> MSEQDEVPSEDRRKYEFRKVIEELKDYEGSGTQLVTIYI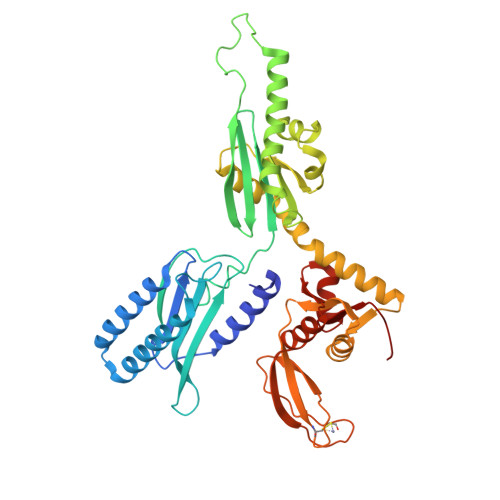PPDKQISDVVAHVTQEHSEASNIKSKQTRTNVQDALTSIKDRLRYYDTFPPDNGMVVFSGAVDSGGGRTDMVTEVLESPPQPIESFRYHCDSAFLTEPLAEMLGDKGLYGLIVLDRRESNVGWLKGKRVQPVKSAESLVPGKQRKGGQSAQRFARLRLEAIDNFYQEVAGMADDLFVPKRHEIDGILVGGPSPTKDEFLDGDYLHHELQDKVLGKFDVSYTDESGLSDLVDAGQAALAEADLMDDKSDMEEFFEELNGGKLATYGFEQTRRNLIMGSVDRLLVSEDLREDVVIYECPNDHEEYETIDRRNTSPEHTCSDCGEEATEVDREDAIDHLMSIADQRGTETHFISTDFEKGEQLLTAFGGYAGILRYSTGV> MLPPDILQNGEFETIYFQTNPTYIKSPIHIPKSTLGKPDTVKIRHFFALLHQDLVVLGLEVFVYLQIYSDFVEKYVYVSKCDTVGLEKSTIKIGKVIGPVLQYIINYNGYKIKMKNLDEKSKDLSDPSTLVRLQRLRDKLPDIYPNLPYYN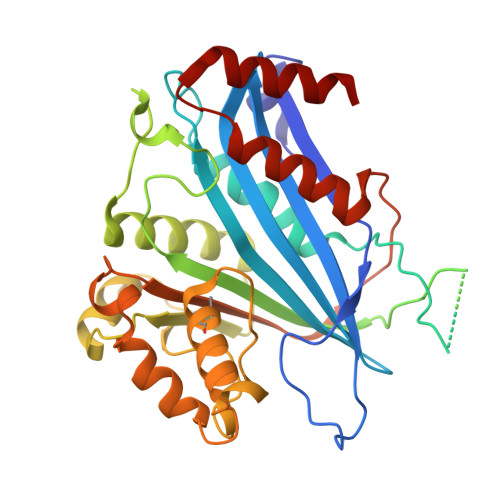DIPPKEECIEYRTLPKTQNLRLCVATKPAKEYLFPNSAKNPYKNLLNGQSLLRWWISIIDSITKGWNNHKLMIPGADKYATRKFIEKYSDWSEGHIFKKDGLAVQAIPLFPDDPKGRFLELVIVECRYGKMTVSRFYQELAYRQEFLLGDCVSLIGCCKENLEVTYHDDLVSTVTISEYKEFMNLLKLVDFSDRVEVSNFVSNYRKSK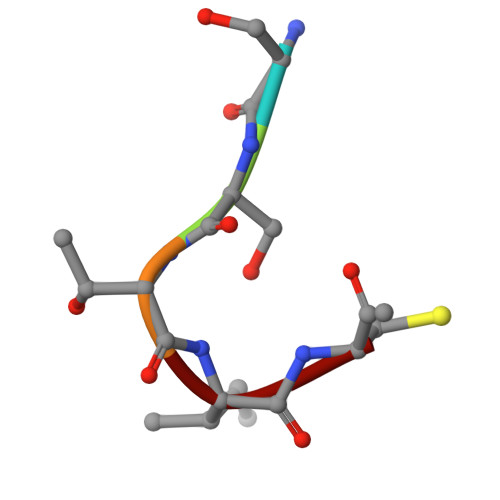> SSTIC>MSLRTAKTGMLLVMVSNIANPFCAAVVKGIEKTAEKNGYRILLCNTESDLARSRSCLTLLSGKMVDGVITMDALSELPELQNIIGAFPWVQCAEYDPLSTVSSVSIDDVAASEYVVDQLVK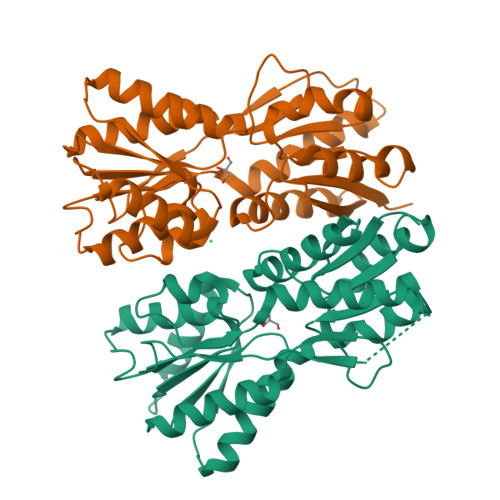SGKKRIALINHDLAYQYAQHRESGYLNRLKFHGLDYSRISYAENLDYMAGKLATFSLLKSAVKPDAIFAISDVLAAGAIQALTESGLSIPQDVAVVGFDGVDISQITVPALTTVQQPSEQIGMKAVSLLLEQIHSDVLAKTVHHLLPWKFVRRQSSEGHHHHHH[2x]>[2x]MRGSHHHHHHGSMQILLANPRGFCAGVDRAISIVENALAIYGAPIYVRH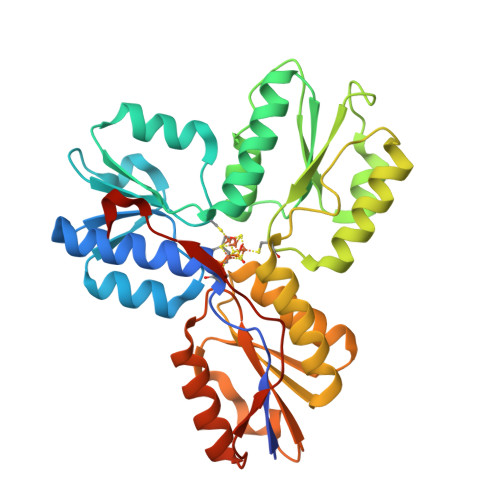EVVHNRYVVDSLRERGAIFIEQISEVPDGAILIFSAHGVSQAVRNEAKSRDLTVFDATCPLVTKVHMEVARASRRGEESILIGHAGHPEVEGTMGQYSNPEGGMYLVESPDDVWKLTVKNEEKLSFMTQTTLSVDDTSDVIDALRKRFPKIVGPRKDDICYATTNRQEAVRALAEQAEVVLVVGSKNSSNSNRLAELAQRMGKRAFLIDDAKDIQEEWVKEVKCVGVTAGASAPDILVQNVVARLQQLGGGEAIPLEGREENIVFEVPKELRVDIREV>MRGSHHHHHHGSACELGTPNMSEEVSKNLSETLFVKHKQAKETSALTQYMPTSQSLLDEIKEKNGFSWYRNLRRLQWVWQGVDPIE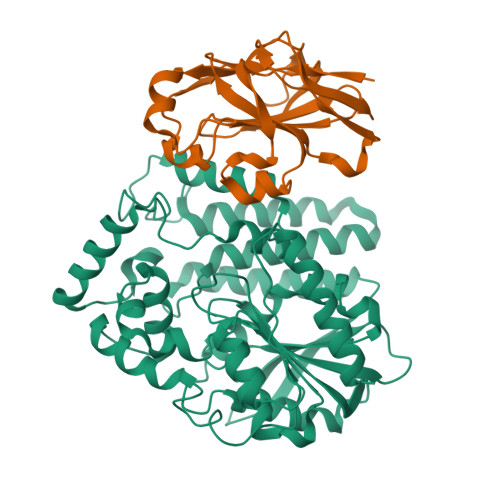QEQVLARIASSKHSRTDEQWLDTVMGYHSGNWAYEWTRLGMEHQKRAGEMTNEAASEALFSASLCYSIAGYPHLKSDNLAIQAQVLANSAYLEAAKKSKYIIKQLEIPFEKGKITAHLHLTNTDKPHPVVIVSAGLDSLQTDMWRLFRDHLAKHDIAMLTVDMPSVGYSSKYPLTEDYSRLHQAVLNELFSIPYVDHHRVGLIGFRFGGNAMVRLSFLEQEKIKACVILGAPIHDIFASPQKLQQMPKMYLDVLASRLGKSVVDIYSLSGQMAAWSLKVQGFLSSRKTKVPILAMSLEGDPVSPYSDNQMVAFFSTYGKAKKISSKTITQGYEQSLDLAIKWLEDELLR[4x];>MRGSHHHHHHGSDTMGLFDKLKKLVSDDSASAGAIEIIAPLSGEIVNIEDVPDVVFAEKIVGDGIAIKPTGNKMVAPVNGTIGKIFETNHAFSIESDDGVELFVHFGIDTVELKGEGFTRIAEEGQTVKAGDTVIEFDLALLEEKAKSTLTPVVISNMDEIKELNKLSGSVVVGETPVLRVTK[4x]> MSAIENFDAHTPMMQQYLRLKAQHPEILLFYRMGDFYELFYDDAKRASQLLDISLTKRGASAGEPIPMAGIPYHAVENYLAKLVNQGESVAICEQIGDPATSKGPVERKVVRIVTPGTISDEALLQERQDNLLAAIWQDSKGFGYATLDISSGRFRLSEPADRETMAAELQRTNPAELLYAEDFAEMSLIEGRRGLRRRPLWEFEIDTARQQLNLQFGTRDLVGFGVENAPRGLCAAGCLLQYAKDTQRTTLPHIRSITMEREQDSIIMDAATRRNLEITQNLAGGAENTLASVLDCTVTPMGSRMLKRWLHMPVRDTRV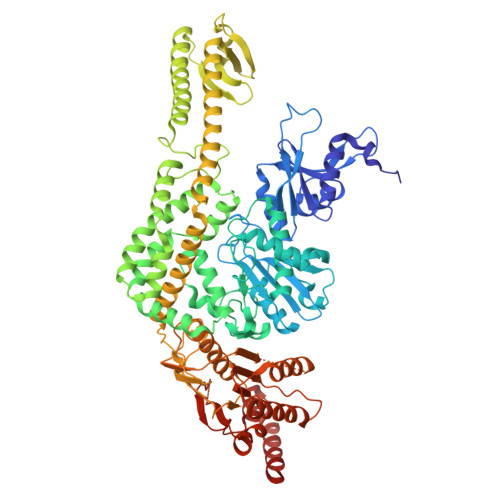LLERQQTIGALQDFTAGLQPVLRQVGDLERILARLALRTARPRDLARMRHAFQQLPELRAQLETVDSAPVQALREKMGEFAELRDLLERAIIDTPPVLVRDGGVIASGYNEELDEWRALADGATDYLERLEVRERERTGLDTLKVGFNAVHGYYIQISRGQSHLAPINYMRRQTLKNAERYIIPELKEYEDKVLTSKGKALALEKQLYEELFDLLLPHLEALQQSASALAELDVLVNLAERAYTLNYTCPTFIDKPGIRITEGRHPVVEQVLNEPFIANPLNLSPQRRMLIITGPNMGGKSTYMRQTALIALMAYIGSYVPAQKVEIGPIDRIFTRVGAADDLASGRSTFMVEMTETANILHNATEYSLVLMDEIGRGTSTYDGLSLAWACAENLANKIKALTLFATHYFELTQLPEKMEGVANVHLDALEHGDTIAFMHSVQDGAASKSYGLAVAALAGVPKEVIKRARQKLRELESIS>VRSSSRTPSDKPVAHVVANPQAEGQLQWLNRRANALLANGVELRDNQLVVPSEGLYLIYSQVLFKGQGCPSTHV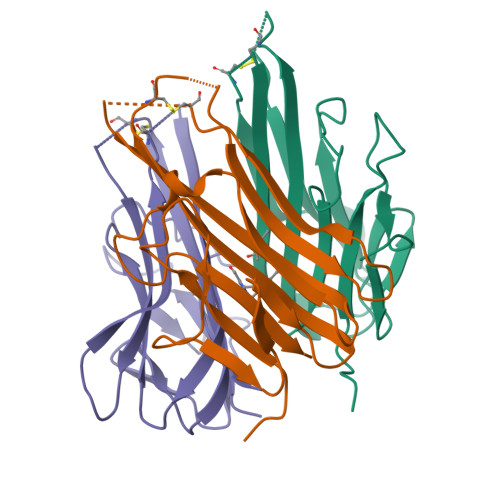LLTHTISRIAVSYQTKVNLLSAIKSPCQRETPEGAEAKPWYEPIYLGGVFQLEKGDRLSAEINRPDYLDFAESGQVYFGIIAL[3x]> MNGTQASNGVLHLDALIIGSGFSGIYLLHKLRDELKLKVKIFEAESDIGGTWNNNRYPGARVDCPVPFYAYSLPEVWQSWNWTELYPNQKEIKSYFDHVDRVLDVRKDCLFHSRVNEGTFDEATGRWTVWTTDGKVATAKYLLVAVGFASKSYLPDWKGLDSFKGTIYHSAHWPEAEEISVKGKKVAVIGTGSTGIQIFQEWAREAEEAFLFQRTPNLCLPMRQQELHAGYQVKDKGEYADYLAECALTFGGLEYQQTPKNTFDASEEEREAFWEDLYQMGGFRFWQNNYQDLLTSLDANREAYNFWARKTRARIQDPKKRDLLAPLEPPYPFGTKRPSLEQDFYEQFNKSNVHIVDTKSQPIVGVTPTGIVTADEKVHEVDIIAVATGFDAVTGGLLRLGLKDVNGVGLDERWKDGMSTYLGMAISGFPNMFLPYSLQAPTAFANGPTLIELQGDWITSLIRKMEMENVQSVTATPHAESAWNDEVNMIANKTLLPLTDSWYMGSNIPGKPVQSLNYLGGLPTYRERCAKVLDEDFFGFAKAHHHHHH

Baeyer-Villiger monooxygenases (BVMOs) are flavin-dependent enzymes that catalyze the conversion of ketones to esters using NAD(P)H and molecular oxygen. In addition to this typical reaction, they can also catalyze heteroatom oxidation, including sulfoxidation and N-oxidation, as well as epoxidation reactions. Amongst the four BVMOs described, BVMOAFL838 showed the best conversion of alkanones with chain lengths of C8-C12, but was unable to convert most of the cyclic ketones tested. BVMOAFL838 has a clear preference towards aliphatic ketones and phenyl substituted 2-alkanones (aryl ketones where the alkyl chain is at least two carbons between the phenyl and carbonyl group).

The crystal structure of BVMOAFL838, the first of a fungal BVMO, was determined at a resolution of 1.9 Å. Despite numerous attempts to co-crystallize BVMOAFL838 with co-factor and substrates, none of the crystals analyzed showed any electron density for bound NADP+ or the substrates used. BVMOAFL838, similar to the four bacterial BVMOs, displays two Rossmann fold domains, representing the FAD and NADP binding domains, with the isoalloxazine ring of FAD positioned at the domain interface. The FAD is bound with the re-face exposed to the substrate binding pocket and the si-face on top of a conserved Tyr69 and Trp52 forming conserved hydrogen bond interactions with the ribitol moiety of FAD. The catalytic site Arg337 and Asp63, implicated in stabilization of the peroxyflavin intermediate and positioning and guiding the cofactor and substrate during catalysis, are conserved. The Arg is located in the “in” position and forms two salt bridges with Asp. Similar to PAMO, a bulge (residues 442–444) protrudes into the active site of BVMOAFL838. Partially covering the substrate entry channel of BVMOAFL838 is a loop region (residues 449 to 514) of which the first half forms an α-helix structure. In BVMOAFL838 the mobile/“variable” loop adopts a position similar to that in the CHMO “closed” structure, where part of the active site entry channel is closed off. In this conformation however, the conserved Trp502 (W492 CHMO numbering) is positioned away from the active site and the NADPH cofactor, suggesting a rearrangement of this loop upon cofactor and substrate binding.> MGSSHHHHHHSQDPNSMPDNTIQWDKDADGIVTLTMDDPSGSTNVMNEAYIESMGKAVDRLVAEKDSITGVVVASAKKTFFAGGDVKTMIQARPEDAGDVFNTVETIKRQLRTLETLGKPVVAAINGAALGGGLEIALACHHRIAADVKGSQLGLPAVTLGLLPGGGGVTRTVRMFGIQNAFVSVLAQGTRFKPAKAKEIGLVDELVATVEELVPAAKAWIKEELKANPDGAGVQPWDKKGYKMPGGTPSSPGLAAILPSFPSNLRKQLKGAPMPAPRAILAAAVEGAQVDFDTASRIESRYFASLVTGQVAKNMMQAFFFDLQAINAGGSRPEGIGKTPIKRIGVLGAGMMGAGIAYVSAKAGYE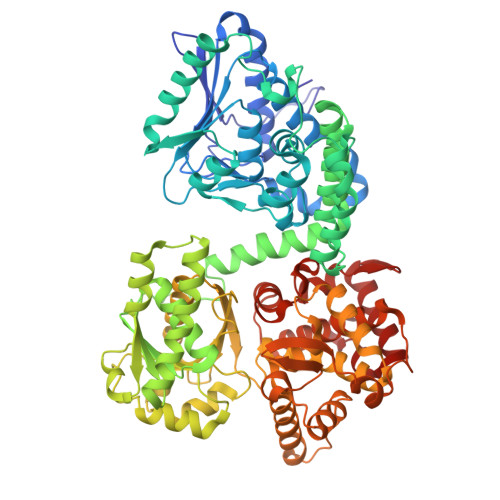VVLKDVSLEAAAKGKGYSEKLEAKALERGRTTQERSDALLARITPTADAADFKGVDFVIEAVFENQELKHKVFGEIEDIVEPNAILGSNTSTLPITGLATGVKRQEDFIGIHFFSPVDKMPLVEIIKGEKTSDEALARVFDYTLAIGKTPIVVNDSRGFFTSRVIGTFVNEALAMLGEGVEPASIEQAGSQAGYPAPPLQLSDELNLELMHKIAVATRKGVEDAGGTYQPHPAEAVVEKMIELGRSGRLKGAGFYEYADGKRSGLWPGLRETFKSGSSQPPLQDMIDRMLFAEALETQKCLDEGVLTSTADANIGSIMGIGFPPWTGGSAQFIVGYSGPAGTGKAAFVARARELAAAYGDRFLPPESLLS> GSHMDGTEKWRFKTNKAIESTPVIGNDGTIYFGSNHLYAINPDGTEKWNFYAGYWTVTRPAISEDGTIYVTSLDGHLYAINPDGTEKWRFKTGKRIESSPVIGNTDTIYFGSYDGHLYAINPDGTEKWRFKTNKAIESTPVIGNDGTIYFGSNHLYAINPDGTEKWNFYAGYWTVTRPAISED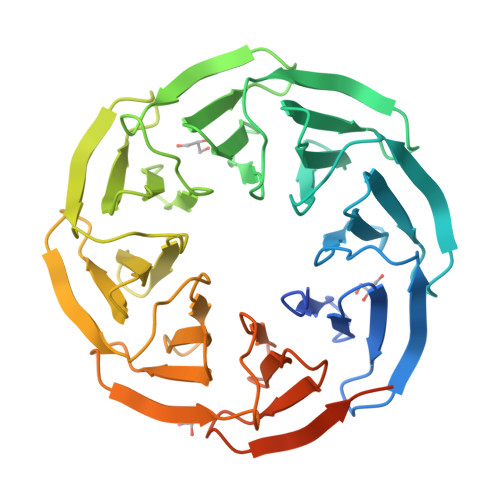GTIYVTSLDGHLYAINPDGTEKWRFKTGKRIESSPVIGNTDTIYFGSYDGHLYAINPDGTEKWRFKTNKAIESTPVIGNDGTIYFGSNHLYAINPDGTEKWNFYAGYWTVTRPAISEDGTIYVTSLDGHLYAINPDGTEKWRFKTGKRIESSPVIGNTDTIYFGSYDGHLYAINP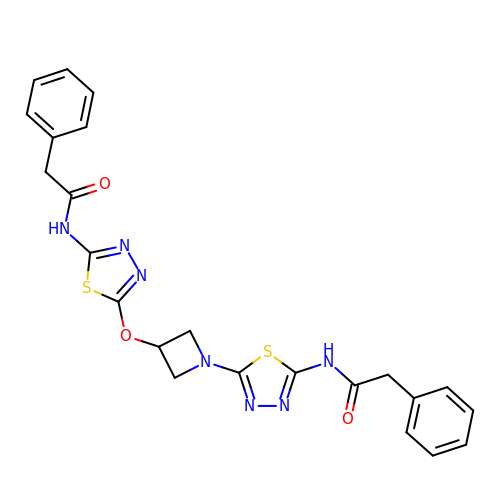2-phenyl-N-{5-[(1-{5-[(phenylacetyl)amino]-1,3,4-thiadiazol-2-yl}azetidin-3-yl)oxy]-1,3,4-thiadiazol-2-yl}acetamide | C23 H21 N7 O3 S2 | GBCGCMNKHTXFKN-UHFFFAOYSA-N>[4x]GETQPESAAFTAPSTDNPIRINFNENPLGMSPKAQAAARDAVVKANRYAKNEILMLGNKLAAHHQVEAPSILLTAGSSEGIRAAIEAYASLEAQLVIPELTYGDGEHFAKIAGMKVTKVKMLDNWAFDIEGLKAAVAAYSGPSIVYLVNPNNPTGTITPADVIEPWIASKPANTMFIVDEAYAEFVNDPRFRSISPMITQGAENIILLKTFSKIHAMAGMRVGYAVAHPTVIALMGRYVAGEKI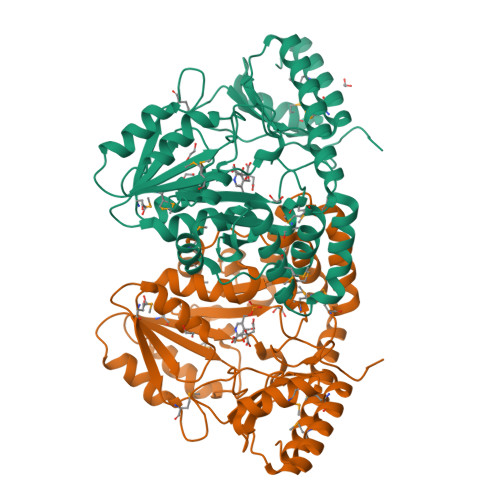NFSGVDAALASMNDSAFITYSKKSNDVSRQILLKALEDLKLPYLPSEGNFVFHQLVVPLKDYQTHMADAGVLIGRAFPPADNWCRISLGTPQEMQWVADTMREFRKKSWI> MMRTVQLRTLRPCIRAQQQPVRPSTS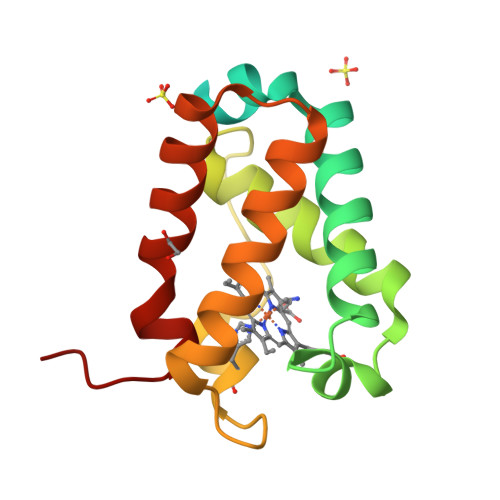ATAAAATAPAPARKCPSSLFAKLGGREAVEAAVDKFYNKIVADPTVSTYFSNTDMKVQRSKQFAFLAYALGGASEWKGKDMRTAHKDLVPHLSDVHFQAVARHLSDTLTELGVPPEDITDAMAVVASTRTEVLNMPQQ> SNAMEVTVPATLNVLNGSDARLPCTFNSAYTVNHKQFSLNWTYQECNNCSEEMFLQFRMKIINLKLERFQDRVEFSGNPSKYDVSVMLRNVQPEDEGIYNCYIMNPPDRHRGHGKIHL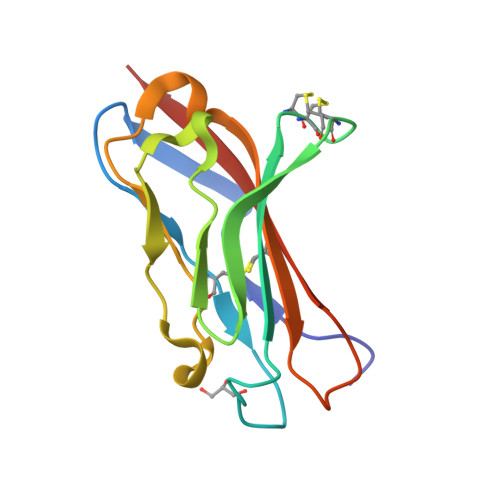QVLMEEP In this paper we describe the first crystal structure of CNMT, an essential enzyme in the core pathway to BIAs, which introduces the amino methyl functionality that is often essential for the bioactivity of most of the medically important BIAs. Previous studies with CNMT from Coptis japonica showed that this S‐adenosyl‐l‐methionine (AdoMet) dependent enzyme can N‐methylate a number of natural THIQ, exhibiting highest activity with coclaurine 4 and heliamine 8.8 To further characterize this enzyme, the C. japonica CNMT was overproduced in E. coli. The CNMT structure reveals a typical class I methyltransferase α/β Rossmann fold forming the AdoMet‐binding domain, which is capped by a predominantly alpha helical BIA substrate recognition domain. CNMT forms a dimeric interface made up of 13 hydrogen bonds and 3 salt bridges, similar to that seen in the PavNMT structure.

CNMT consists of a relatively smaller, more compact, active site (CNMT 387 Å2/PavNMT 1081 Å2) which is shaped by positioning an extended loop (residues 249–260) and residues 64–82 of helix α4 closer to the substrate binding pocket. Three active site residues, E204, E207 and H208 are in close proximity to the methyl group of the product 8 a in the CNMT structure. Consequently, E204, E207, and H208 could potentially stabilize the substrate ammonium ion through H‐bonding or a salt bridge. Given that the E207 carboxyl is 7 Å from H208 imidazole, which is in turn 5 Å from the N atom of 8 a in the CNMT structure, H208 and E207 may function as a catalytic diad. Moreover, the backbone carbonyl group of T261 is within H‐bonding distance of H208, which could similarly assist H208 in functioning as a general base. The close proximity of E204 carboxyl to the N atom of 8 a (4 Å) suggest that E204 may interact electrostatically with the substrate/product ammonium ion. The proximity of the residues Y328, W329, R330, G331, and F332 to 8 a also indicates these residues may be involved in substrate binding. The fact that F332 is closer to the product 8 a, in the CNMT structure, than W329, would also support this hypothesis. The CNMT structure indicates that larger substituents at C3 or C4 would clash with E204, E207, H208, and I234 residues of the CNMT active site. The structure of CNMT with 9 is very similar to the N‐methylheliamine 8 a structure except the two ligands are flipped relative to one another in the active site, with the carbonyl group of 9 in the same position as the amino group of 8 a.

>[2x]QTKKAAIVELLKQLELGLVPYDDIKQLIRRELARRLQWGYKPTYEEQIAEIQNLTHSLRQMKIATEVETLDSQLYEIPIEFLKIMNGSNLKGSCCYFKEDSTTLDEAEIAMLDLYCERAQIQDGQSVLDLGCGQGALTLHVAQKYKNCRVTAVTNSVSQKEYIEEESRRRNLLNVEVKLADITTHEMAETYDRILVIELFEHMKNYELLLRKISEWISKDGLLFLEHICHKTFAYHYEPLDDDDWFTEYVFPAGTMIIPSASFFLYFQDDVSVVNHWTLSGKHFSRTNEEWLKRLDANLDVIKPMFETLMGNEEEAVKLINYWRGFCLSGMEMFGYNNGEEWMASHVLFKK>MGSSHHHHHHSSGETVRFQGHMELTPDQQTLLHFIMDSY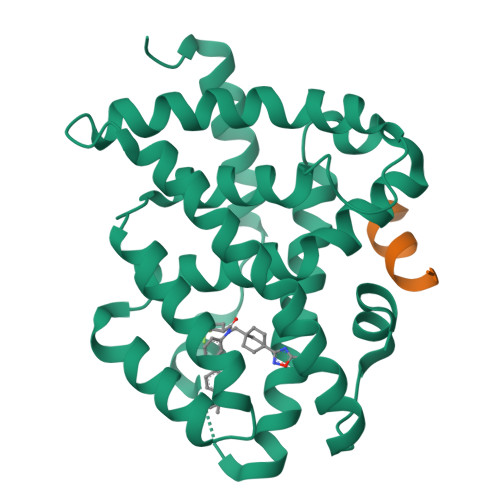NKQRMPQEITNKILKEAFSAEENFLILTEMATNHVQVLVEFTKKLPGFQTLDHEDQIALLKGSAVEAMFLRSAEIFNKKLPSGHSDLLEARIRNSGISDEYITPMFSFYKSIGELKMTQEEYALLTAIVILSPDRQYIKDREAVEKLQEPLLDVLQKLCKIHQPENPQHFACLLGRLTELRTFNHHHAEMLMSWRVNDHKFTPLLCEIWDVQ[2x];>[2x]KDHQLLRYLLDKDE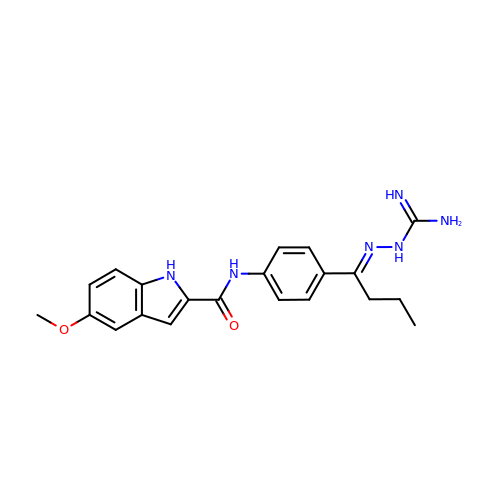N-{4-[(1E)-N-carbamimidoylbutanehydrazonoyl]phenyl}-5-methoxy-1H-indole-2-carboxamide | C21 H24 N6 O2 | IFLKHYHIUCIDRM-NLRVBDNBSA-N>MKSLIFTLSLLALTGCTITRQAQVSEASPISGIVRLTYNQPLFFTSRTDDYVSHGTATRECQQMGYADAVSFGQPVGTCSIYAGSLCLNTRFTLSWQCRGVAVPQIMPLYY[26x];>MQKYALHAYPVMALMVATLTGCAWIPAKPLVQGATTAQPIPGPVPVANGSIFQSAQPINYGYQPLFEDRRPRNIGDTLTIVLQENVSASKSSSANASRDGKTSFGFDTVPRYLQGLFGNSRADMEASGGNSFNGKGGANASNTFSGTLTVTVDQVLANGNLHVVGEKQIAINQGTEFIRFSGVVNPRTISGSNSVPSTQVADARIEYVGNGYINEAQNMGWLQRFFLNLSPM[26x];>[26x]MFKALAGIVLALVATLAHAERIRDLTSVQGVRENSLIGYGLVVGLDGTGDQTTQTPFTTQTLNNMLSQLGITVPTGTNMQLKNVAAVMVTASYPPFARQGQTIDVVVSSMGNAKSLRGGTLLMTPLKGVDSQVYALAQ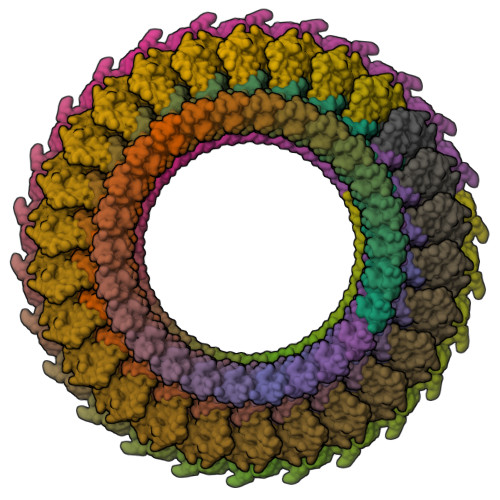GNILVGGAGASAGGSSVQVNQLNGGRITNGAIIERELPTQFGAGNTINLQLNDEDFTMAQQITDAINRARGYGSATALDARTVQVRVPSGNSSQVRFLADIQNMEVNVTPQDAKVVINSRTGSVVMNREVTLDSCAVAQGNLSVTVNRQLNVNQPNTPFGGGQTVVTPQTQIDLRQSGGSLQSVRSSANLNSVVRALNALGATPMDLMSILQSMQSAGCLRAKLEII>[4x]MAHTGRMFKIEAAEIVVARLPLKFRFETSFGVQTHKVVPLLILHGEGVQGVAEGTMEARPMYREETIAGALDLLRGTFLPAILGQTFANPEAVSDALGSYRG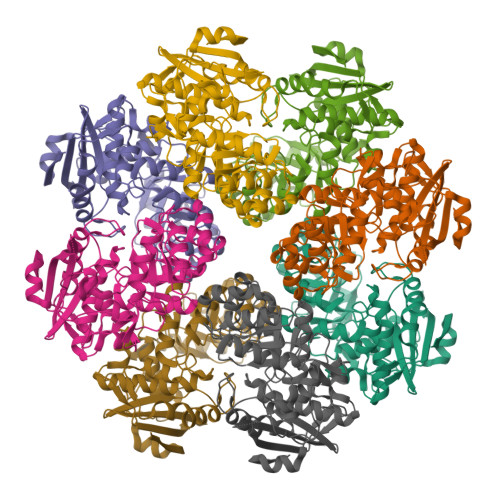NRMARAMVEMAAWDLWARTLGVPLCTLLGGHKEQVEVGVSLGIQADEQATVDLVRRHVEQGYRRIKLKIKPGWDVQPVRATREAFPDIRLTVDANSAYTLADAGRLRQLDEYDLTYIEQPLAWDDLVDHAELARRIRTPLCLDESVASASDARKALALGAGGVINLKVARVGGHAESRRVHDVAQSFGAPVWCGGMLESGIGRAHNIHLSCLSNFRLPGDTSSASRYWERDLIQEPLEAVDGLMPVPQGPGTGVTLDREFLATVTEAQEEHRA> EVPQMTSSSAPDLEEEDDYTAYAPLTCYFTNSTLGLLAPPNCSVL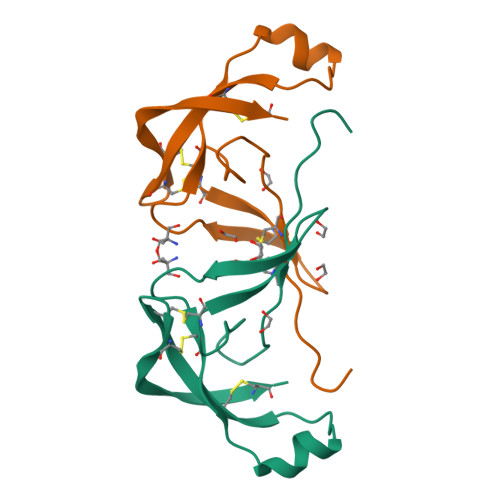CNSTTTWFNETSPNNASCLLTVDFLTQDAILQENQPYNCSVGHCDNGTCAGPPRHAQCW> MAPITAYSQQTRGLLGCIITSLTGRDKNQV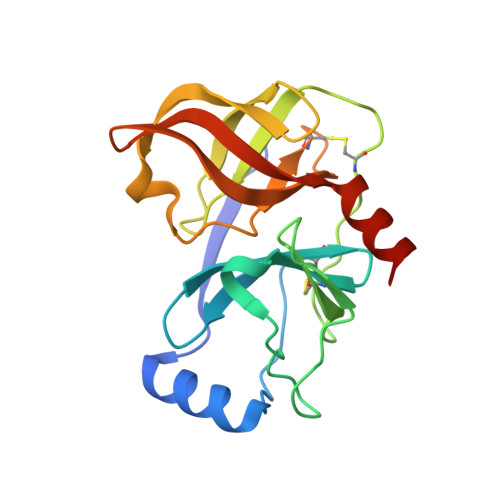DGEVQVLSTATQSFLATCVNGVCWTVYHGAGSKTLAGPKGPITQMYTNVDQDLVGWPAPPGARSMTPCTCGSSDLYLVTRHADVIPVRRRGDSRGSLLSPRPVSYLKGSSGGPLLCPSGHVVGIFRAAVCTRGVAKAVDFIPVESMETTMRASKKKK> AGMAHAASYLSVGYFNGGGDVTAGPGGDINKLDVTQITHLNYSFGLIYNDEKQETNPALKDPSRLHQIYLSPKVMADLQLLPVLRKQNPELKVLLSVGGWGARGFSGAAATAESRAVFIRSVQQVIKQYHLDGIDLDWEYPVNGAWGLVESQPADRANFTLLLAELHKALDKGKLLTIAVGANVKSPQEWVDVKGIAPYLDYINLMTYDMAYGTQYFNSNLYDSKQWPTVAAA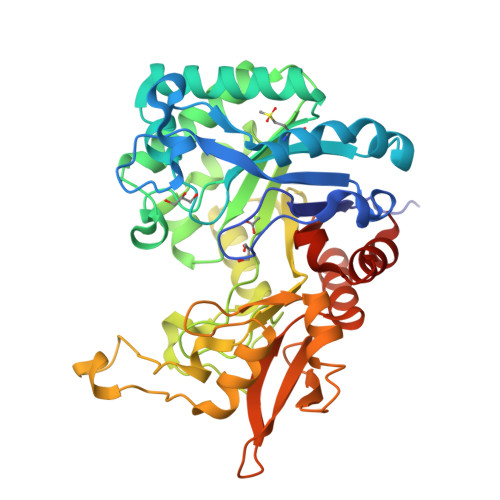DRYSANFVVDNYLAAGLKPAQLNLGIGFYGRVPKRATEPGIDWDKADAAKNPVTQPYFTARETAVFKAMGLDLTKDSYFKYNDIVSKLLNDPQRRFTAHWDSDAQVPYLTMKSAEGKPLFAISYENPRSVALKADYIKSKGLGGAMFWEYGADDNNRLAHQLAESLGINGGKQ>[4x]GSHMIVYQTLNPTTETVERSFDLHTPAQMKDITDRAEHVWKTDWKLRSIAQRKEIVSRAADLLRRDRQHHASLIATEMGKALPDALEEIDVTADILSFYANGAEEFLAPTPLKVKTGQAKIINQPLGIIYCIEPWNFPYYQLARVAGPNLMAGNVVIAKHAPNVPQCALAFEKLFHDAGAPVGAYANIFLDNDQSAELIKDERIRGVALTGSERAGQAVAAQAGAALKKDT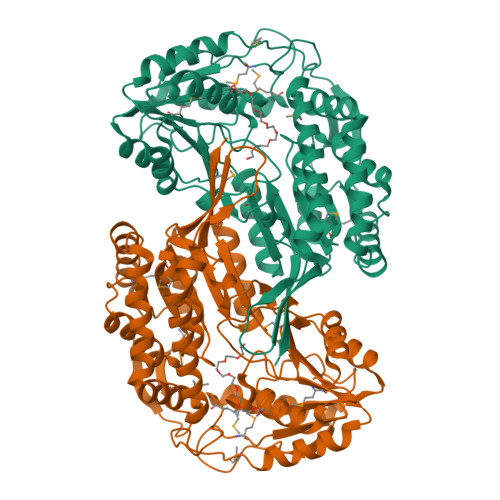MELGGSDAFIVLDDADLDLAVKWAVWGRFANNGQVCTAAKRMIVHEKVYDAFLDGLKTAITRFRIGNPLDRDTTHGPMSSLRAMELALDQTAEAVKGGATLVAGGKRMDRKGFFMEPTILTDVSKDNPVFYQEIFGPVAVVHKVASEQAAIDLANDSPYGLGGAVFSRDIARAEKVAEQVETGMVFINTATAAAPELPFGGIKNSGFGRELSFLGIEEFINRKLVRIG> MSWQEKINAALDARGAADALRRRYPVAQGAGRWLVADDRQYLNFSSNDYLGLSHHPQIIRAWQQGAEQFGIGSGGSGHVS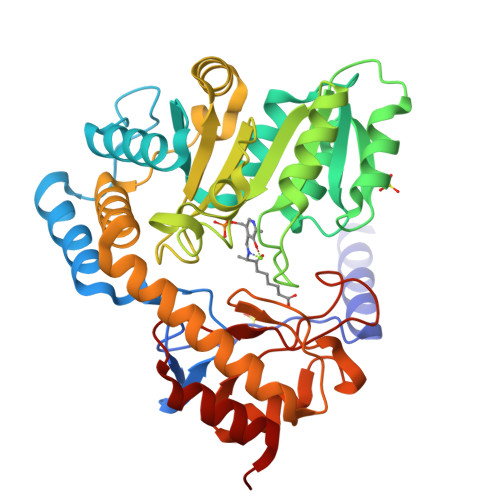GYSVVHQALEEELAEWLGYSRALLFISGFAANQAVIAAMMAKEDRIAADRLSHASLLEAASLSPSQLRRFAHNDVTHLARLLASPCPGQQMVVTEGVFSMDGDSAPLAEIQQVTQQHNGWLMVDDAHGTGVIGEQGRGSCWLQKVKPELLVVTFGKGFGVSGAAVLCSSTVADYLLQFARHLIYSTSMPPAQAQALRASLAVIRSDEGDARREKLAALITRFRAGVQDLPFTLADSCSAIQPLIVGDNSRALQLAEKLRQQGCWVTGIRPPTVPAGIARLRLTLTAAHEMQDIDRLLEVLHGNG>[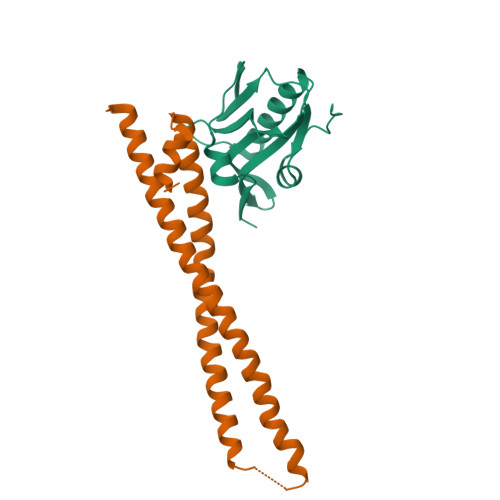2x]ASRYLTDMTLEEMSRDWFMLMPKQKVAGSLCIRMDQAIMDKNIILKANFSVIFDRLETLILLRAFTEEGAIVGEISPLPSLPGHTDEDVKNAVGVLIGGLERNDNTVRVSETLQRFAWRSSNENGRPPLPPKQKRKMARTIKSEV;>[2x]GSKEDSVEAVGAQLKVYHQQYQDKSREYDQLYEEYTRTSQELQMKRTAIEAFNETIKIFEEQGQTQEKSSKEYLERFRREGNEKEMQRILLNSERLKSRIAEIHESRTKLEQQLRAQASDNREIDKRMNSLKPDLMQLRKIRDQYLVWLTQKGARQKKINEWLGI> SNAPPGTVDKKMVEKCWKLMDKVVRLCQNPKLALKNSPPYILDLLPDTYQHLRTILSRYEGKMETLGENEYFRVFMENLMKKTKQTISLFKEGKERMYEENSQPRRNLTKLSLIFSHMLAELKGIFPSGLFQGDTFRITKADAAEFWRKAFGEKTIVPWKSFRQALHEVHPISSGLEAMALKSTIDLTCNDYISVFEFDIFTRLFQPWSSLLRNWNSLA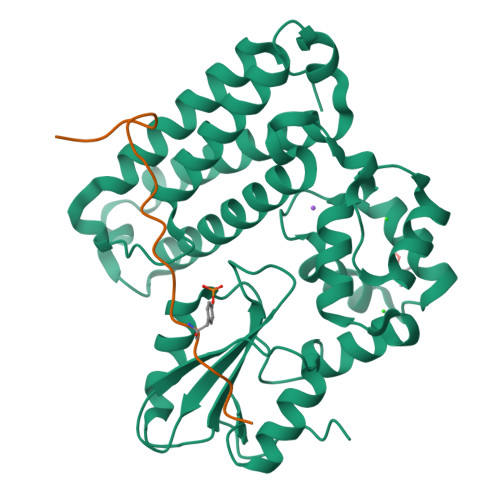VTHPGYMAFLTYDEVKARLQKFIHKPGSYIFRLSCTRLGQWAIGYVTADGNILQTIPHNKPLFQALIDGFREGFYLFPDGRNQNPDLTG;> XQQVHVLSLDQIRAIRNTNEYTEGPT> APVAFPQDRTCPYDPPTAYDPLREGRPLSRVSLYDGRSVWVVTGHAAARALLSDQRLSSDRTLPRFPATTERFEAVRTRRVALLGVDDPEHRTQRRMLVPSFTLKRAAALRPRIQETVDGLLDAMEAQGPPAELVSAFALPLPSMVICALLGVPYADHDFFESQSRRLLRGPGIAEVQDARAQLDDYLYALIDRKRKEPGDGLLDDLIQEQLNRGTVDRAELVSLATLLLIAGHETTANMISLGTFTLLRHPEQLAELRAEPGLMPAAVEELLRFLSIADGLLRVATEDIEVAGTTIRADEGVVFATSVINRDAAGFAEPDALDWHRSARHHV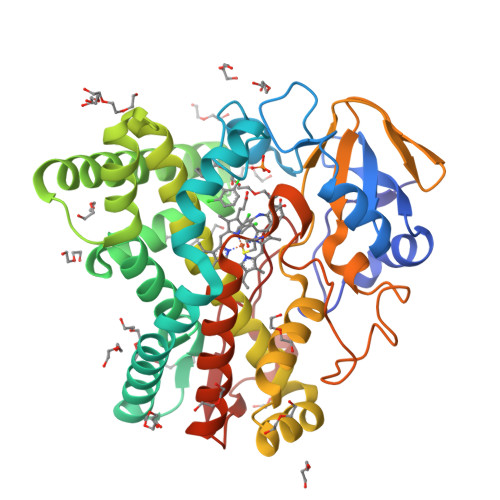AFGFGIHQCLGQNLARAEMEIALGTLFERLPGLRLAAPADEIPFKPGDTIQGMLELPVTW> GSPLPSDVRPPHILVKTLDYIVDNLLTTLPESEGFLWDRMRSIRQDFTYQNYSGPEAVDCNERIVRIHLLILHIMVKSNVEFSLQQELE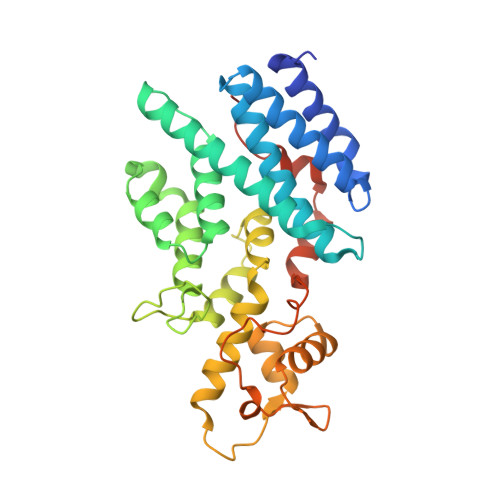QLHKSLITLSEIYDDVRSSGGTCPNEAEFRAYALLSKIRDPQYDENIQRLPKHIFQDKLVQMALCFRRVISNSAYTERGFVKTENCLNFYARFFQLMQSPSLPLLMGFFLQMHLTDIRFYALRALSHTLNKKHKPIPFIYLENMLLFNNRQEIIEFCNYYSIEIINGDAADLKTLQHYSHKLSETQPLKKTYLTCLERRLQKTTYKGLINGGEDNLASSVYVKDPKK> MAKEVIVYTSNTCPHSFTVKEFLSENNVEFTEKNIQTDAAARKELMKKGIMAVPVIQIDEEVVVGFDRDKIEEL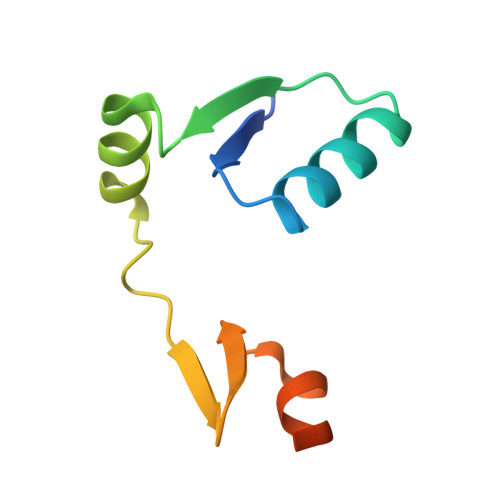LGLEHHHHHH> ESRTSAPSGCLTVGSDGTYSTIGDALDALGSSTSSACIYVAS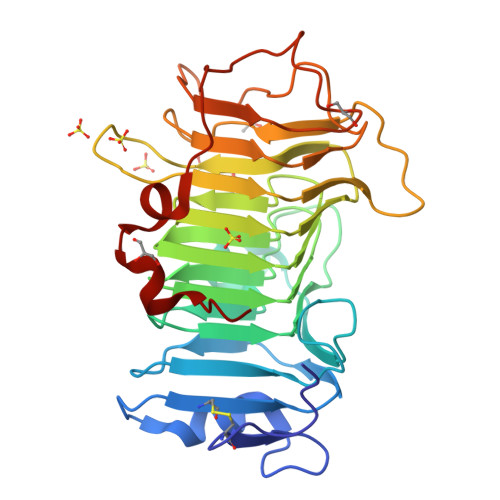GTYEEQLTIDYAGDLTLYGETTDTSTYKDNVVTITHTISSPDAGSLDKSATVNVVSDGFSMYNINVENGYGEGAQAVALVGNADQLGFYGCQFSGYQDTLYVKAGTQYYSNCMIEGAVDYIFGDASVWFGECDIVSNGAGAITASSRETSSDSGWYAIDNCNIKAASGVSLTEEVYLGRPWRVLARVIYQNSVLSDIINPKGWTTMADGATPLYYEYNNSGAGSDTSDREYETSISAAVDKTTVLGETWGDWIDRSY> GPGSEFRNKRATRGTYSPSAQEYCNPRLEMDNV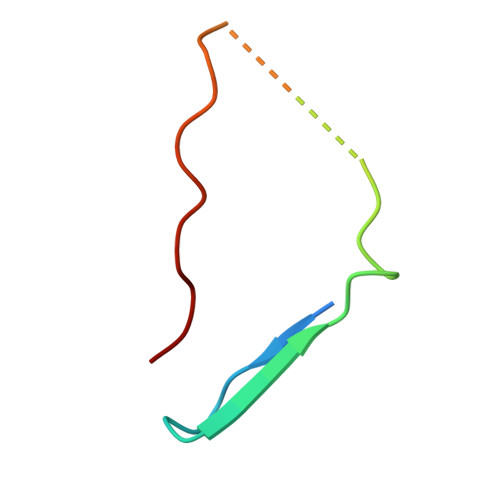LKPPPEERLI Of interest was PixJ from the thermophilic cyanobacterium Thermosynechococcus elongatus (Te), which transitions almost completely between blue light-absorbing Pb and green light-absorbing Pg end states using a phycoviolobilin (PVB) chromophore. In addition to the conventional thioether linkage that connects C522 within the GAF domain to the C31 carbon of the A pyrrole ethylidene side chain, PVB is attached via a second thioether linkage between C494 of the GAF domain and the C10 carbon between the B and C pyrrole rings. The end result is conversion of C10 from sp2 to sp3 hybridization, which shortens the π-conjugation system of PVB and induces the substantial hypsochromic shift from green- to blue-light absorption. Comparisons implied that photoconversion involves isomerization at the C15=C16 bond, a rupture of the C494–C10 thioether linkage, restoration of the π-conjugation between the B and C pyrrole rings, rotation and translation of the bilin in the GAF pocket, and conformational rearrangements of the protein backbone and surrounding amino acid side chains.

To help unravel this photoconversion sequence, we produced a construction of the GAF domain from TePixJ, hereafter called TePixJ(GAF), that enabled production of crystals that retain reversible photoconversion between Pb and Pg as well as thermal reversion from Pg back to Pb. From large-scale crystallization trials of Pb in darkness, we identified conditions at pH 5.5 that would generate yellow rod-shaped crystals. Remarkably, upon irradiation with blue light at room temperature, the crystal color transitioned to magenta, which returned to yellow/brown in darkness, revealing the presence of a photochromic bilin. In an effort to generate a crystal structure of TePixJ(GAF) as Pb with minimal X-ray–induced damage, we used continuous vector translation across the length of the crystals to lessen X-ray dose. The asymmetric unit was occupied by 2 TePixJ(GAF) molecules (designated units A and B), which dimerized in crystallo via a 4-helix bundle involving the α1- and α5-helices. Additionally, the electron density for both PVB moieties and the adjoining thioether linkages were well-resolved and continuous. Superposition of the 2 molecules in the asymmetric unit showed that the main-chain atoms were highly similar throughout (root-mean-square deviation [rmsd] of 0.47 Å for all Cα-atoms) with some differences noticeable at helix α4, which appeared to subtly alter the atomic positions of the adjacent PVB moieties within their binding pockets. As in previous structures, the B-ring propionate of unit A formed hydrogen bonds with H498 and W499. However, this contact was altered in unit B. Although the hydrogen bond with W499 was retained, H498 was displaced by R507′ from unit A in the symmetry-related molecule, which formed a salt bridge with the B-ring propionate of unit B.

>SELRDRQAIFETLVAKGRELLACDRVIVYAFDDNYVGTVVAESVAEGWPQARDQVIEDPCFREHWVEAYRQGRIQATTDIFKAGLTECHLNQLRPLKVRANLVVPMVIDDQLFGLLIAHQASEPRQWQEIEIDQFSELASTGSLVLERLH[2x]>GHMTVEPFRNEPIETFQTEEARRAMREALRRVREEFGRHYPLYIGGEWVDTKERMVSLNPSAPSEVVGTTAKAGKAEAEAALEAAWKAFKTWKDWPQEDRSAL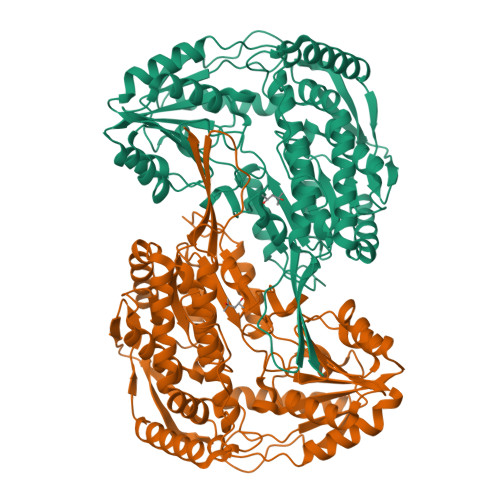LLKAAALMRRRKRELEATLVYEVGKNWVEASADVAEAIDFIEYYARAALRYRYPAVEVVPYPGEDNESFYVPLGAGVVIAPWNFPVAIFTGMIMGPVAVGNTVIAKPAEDAVVVGAKVFEIFHEAGFPPGVVNFLPGVGEEVGAYLVEHPRTRFINFTGSLEVGLKIYEAAGRLAPGQTWFKRAYVETGGKDAIIVDETADFDLAAEGVVVSAYGFQGQKCSAASRLILTQGAYEPVLERVLKRAERLSVGPAEENPDLGPVVSAEQERKVLSYIEIGKNEGQLVLGGKRLEGEGYFIAPTVFTEVPPKARIAQEEIFGPVLSVIRVKDFAEALEVANDTPYGLTGGVYSRKREHLEWARREFHVGNLYFNRKITGALVGVQPFGGFKLSGTNAKTGALDYLRLFLEMKAVAERF[2x]>MGISWLDIYHVVSATVPLYVSMTLGFLSARHLKLFSPEQCAGINKFVAKFSIPLLSFQIISENNPFKMSPKLILSDILQKFLVVVVLAMVLRFWHPTGGRGGKLGWVITGLSISVLPNTLILGMPILSAIYGDEAASILEQIVVLQSLIWYTILLFLFELNAARALPSSGASLEHTGNDQEEANIEDEPKEEEDEEEVAIVRTRSVGTMKILLKAWRKLIINPNTYATLIGIIWATLHFRLGWNLPEMIDKSIHLLSDGGLGMAMFSLGLFMASQSSIIACGTKMAIITMLLKFVLGPALMIASAYCI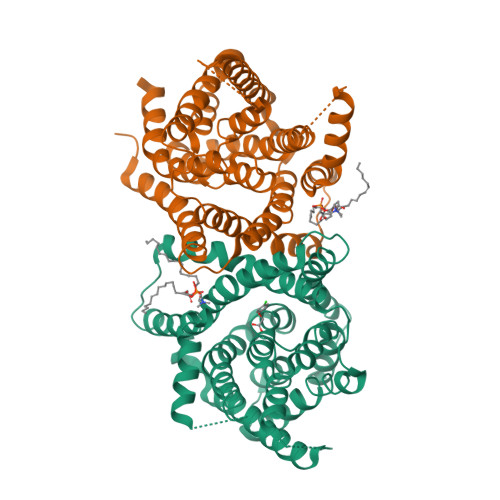RLKSTLFKVAILQAALPQGVVPFVFAKEYNLHPEIISTGVIFGMLIALPTTLAYYFLLDLPGENLYFQ[2x]5-fluoranyl-2-(methylsulfonylamino)benzoic 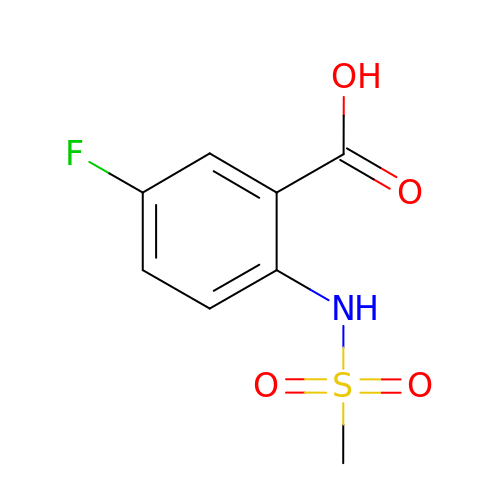acid | C8 H8 F N O4 S | QDIQHFNTURTELA-UHFFFAOYSA-N> KEKLNAFLVHDNVAFYQGDVDTVVNGVDFDFIVNAANENLAHGGGLAKALDVYTKGKLQRLSKEHIGLAGKVKVGTGVMVECDSLRIFNVVGPRKGKHERDLLIKAYNTINNEQGTPLTPIL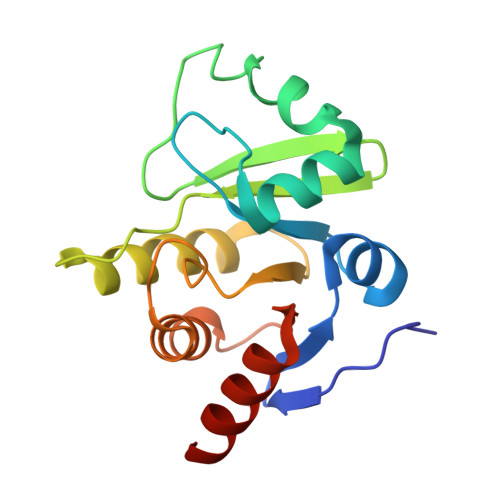SCGIFGIKLETSLEVLLDVCNTKEVKVFVYTDTEVCKVKDFVSGLV> GSHMAQHGALETLKDLAEKEVDDAARLLGEMRRGCQQAEEQLKMLIDYQNEYRSNLNTDMGNGIASNRWIN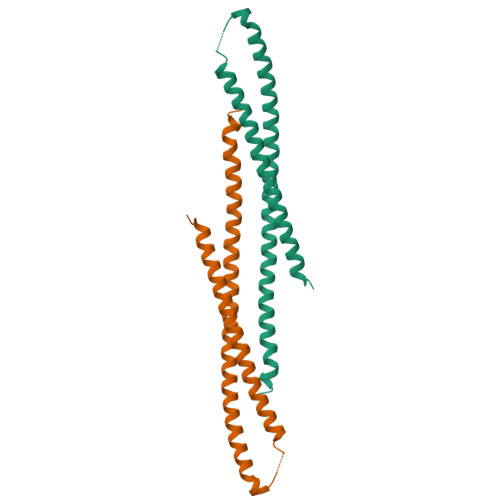YQQFIQTLEKAIEQHRLQLTQWTQKVDLALKSWREKKQRLQAWQTLQDRQTAAALLAENRMDQKKMDEFAQRAAMRKPE> GPVSLQMVTVGHNIALIQPGFSLMNFDGQVFFFGQKGWPKRSCPTGVFHFDIKQNHLKLKPAIFSKDSCYLPPLRYP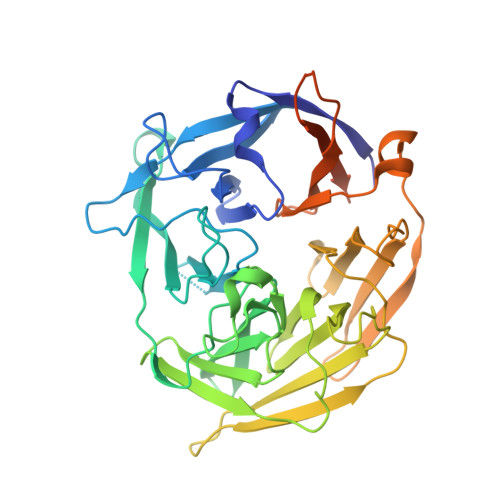ATCSYKGSIDSDKHQYIIHGGKTPNNELSDKIYIMSVACKNNKKVTFRCTEKDLVGDVPEPRYGHSIDVVYSRGKSMGVLFGGRSYMPSTQRTTEKWNSVADCLPHVFLIDFEFGCATSYILPELQDGLSFHVSIARNDTVYILGGHSLASNIRPANLYRIRVDLPLGTPAVNCTVLPGGISVSSAILTQTNNDEFVIVGGYQLENQKRMVCSLVSLGDNTIEISEMETPDWTSDIKHSKIWFGSNMGNGTIFLGIPGDNKQAMSEAFYFYTLRCSEEDLSEDQKIVSNSQTSTEDPGDSTPFEDSEEFCFS>PGIHSGRTRVGKYELGRTLGEGTFAKVKFARNVENGDNVAIKVIDKEKVLKNKMIAQIKREISTMKLIKHPNVIRMFEVMASKTKIYFVLEFVTGGELFDKISSNGRLKEDEARKYFQQLINAVDYCHSRGVYHRDLKPENLLLDANGALKVSDFGLSALPQQVREDGLLHTTCGTPNYVAPEVINNKGYDGAKADLWSCGVILFVLMAGYLPFEDSNLTSLYKKIFKAEFTCPPWFSASAKKLIKRILDPNPATRITFAEVIENEWFKKGYKAPKFENADVSLDDVDAIFDDSGESKNLVVERREEGLKTPVTMNAFELISTSQGLNLGSLFEKQMGLVKRKTRFTSKSSANEIVTKIEAAAAPMGFDVKTNNYKMKLTGEKSGRKGQLAVATEVFQVAPSLYMVEMRKSGGDTLEFHKFYKNLTTGLKDIVWKTIDEEKEEGTDGGGTNGAMANRTIAKQST[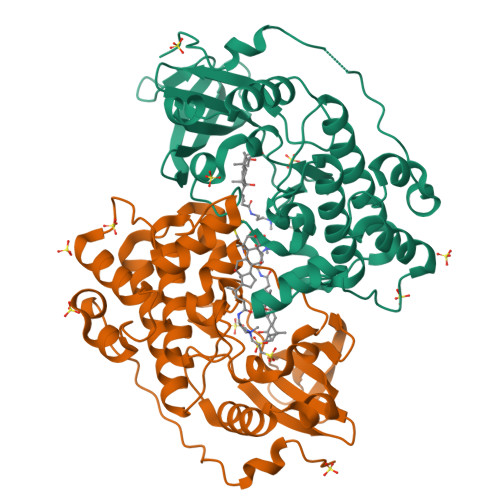4x]>[2x]SELRIILVGKTGTGKSAAGNSILRKQAFESKLGSQT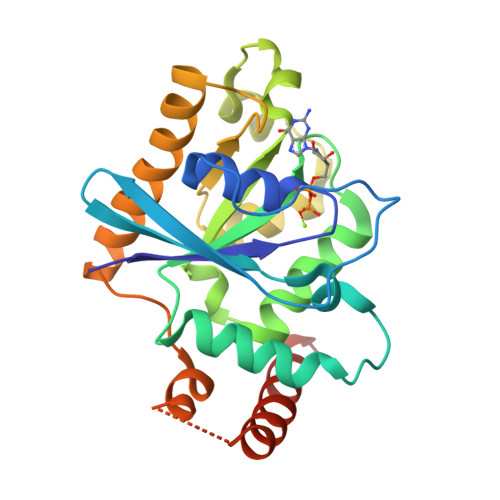LTKTCSKSQGSWGNREIVIIDTPDMFSWKDHCEALYKEVQRCYLLSAPGPHVLLLVTQLGRYTSQDQQAAQRVKEIFGEDAMGHTIVLFTHKEDLNGGSLMDYMHDSDNKALSKLVAACGGRICAFNNRAEGSNQDDQVKELMDCIEDLLMEKNGDHYTNGLYSLIQRSKCGPVGSDERVKEFKQSLIKYMETQRSYTALAEAN LpxA and LpxD are functionally and structurally similar, sharing a homotrimer architecture and conserved active site features, especially in the acyl-chain binding pockets that reside in the dimer interface of the β-helix trimer core. Herein we report the discovery of several small molecules that bind to both P. aeruginosa LpxA and LpxD with μM affinity, identified using a targeted structure-based methodology that utilizes molecular docking, surface plasmon resonance (SPR) bioanalysis, and high-resolution X-ray crystallography.

After failed attempts to crystallize untagged LpxD following protease cleavage, we tested several variations of this LpxD construct by first replacing the thrombin protease cleavage site with a TEV protease recognition sequence, and then excising the first two residues of the LpxD sequence, which are located immediately after the N-terminal 18-AA hexahistidine tag and protease site. The resulting construct led to protein crystals similar to the published one, with each asymmetric unit of the H3 space group containing one monomer that forms a biologically relevant homotrimer through 3-fold crystallographic symmetry operation. Importantly, in the apo structure of the new LpxD construct determined at 1.55 Å resolution, the density of the His-tag linker is no longer observed in the active site. In fact, whereas these residues are ordered in the previous structure, this entire region of the His-tag and protease site is disordered in the current structure. However, our failure to crystallize untagged LpxD suggests the His-tag may still contribute to the stability of the crystal-packing interface, despite the lack of an ordered conformation. An interesting observation in our new LpxD structure is a well-defined magnesium ion in the core of the trimer. This magnesium ion, likely from the crystallization buffer, coordinates six water molecules and appears to be critical to the stability of the crystal, as removing magnesium from the crystallization buffer or chelating the magnesium with EDTA eradicates X-ray diffraction by the crystal. Our new LpxD crystal structures also shed light on a previously uncharacterized magnesium ion at the center of the trimer core. We hypothesize that a magnesium ion can potentially stabilize the trimer.

> MHHHHHHSSGRENLYFQGSTLSYTLGQLAAHVGAEVRGDADLPIQGLATLQEAGPAQLSFLANPQYRKYLPESRAGAVLLTAADADGFAGTALVVANPYLAYASLSHLFDRKPKAAAGIHPTAIVAADAEVDPSASVGAYAVIESGARIGAGVSIGAHCVIGARSVIGEGGWLAPRVTLYHDVTIGARVSIQSGAVIGGEGFGFANEKGVWQKIAQIGGVTIGDDVEIGANTTIDRGALSDTLIGNGVKLDNQIMIAHNVQIGDHTAMAACVGISGSAKIGRHCMLAGGVGLVGHIEICDNVFVTGMTMVTRSITEPGSYSSGTAMQPAAEWKKSAARIRQLDDMARRLQQLEKRLAAVTSSGDASSDA> HHHHHHSSGLEVLFQGPHMASMPEQYRYTLPVKAGEQRLLGELTGAACATLVAEIAERHAGPVVLIAPDMQNALRLHDEISQFTDQMVMNLADWETLPYDSFSPHQDIISSRLSTLYQLPTMQRGVLIVPVNTLMQRVCPHSFLHGHALVMKKGQRLSRDALRTQLDSAGYRHVDQVMEHGEYATRGALLDLFPMGSELPYRLDFFDDEIDSLRVFDVDSQRTLEEVEAINLLPAHEFPTDKAAIELFRSQWRDTFEVKRDPEHIYQQVSKGTLPAGIEYWQPLFFSEPLPPLFSYFPANTLLVNTGDLETSAERFQADTLARFENRGVDPMRPLLPPQSLWLRVDELFSELKNWPRVQLKTEHLPTKAANANLGFQKLPDLAVQAQQKAPLDALRKFLETFDGPVVFSVESEGRREALGELLARIKIAPQRIMRLDEASDRGRYLMIGAAEHGFVDTVRNLALICESDLLGERVARRRQDSRRTINPDTLIRNLAELHIGQPVVHLEHGVGRYAGMTTLEAGGITGEYLMLTYANDAKLYVPVSSLHLISRYAGGAEENAPLHKLGGDAWSRARQKAAEKVRDVAAELLDIYAQRAAKEGFAFKHDREQYQLFCDSFPFETTPDQAQAINAVLSDMCQPLAMDRLVCGDVGFGKTEVAMRAAFLAVDNHKQVAVLVPTTLLAQQHYDNFRDRFANWPVRIEMISRFRSAKEQTQILAEVAEGKIDILIGTHKLLQSDVKFKDLGLLIVDEEHRFGVRHKERIKAMRANVDILTLTATPIPRTLNMAMSGMRDLSIIATPPARRLAVKTFVREYDSMVVREAILREILRGGQVYYLYNDVENIQKAAERLAELVPEARIAIGHGQMRERELERVMNDFHHQRFNVLVCTTIIETGIDIPTANTIIIERADHFGLAQLHQLRGRVGRSHHQAYAWLLTPHPKAMTTDAQKRLEAIASLEDLGAGFALATHDLEIRGAGELLGEEQSGSMETIGFSLYMELLENAVDALKAGREPSLEDLTSQQTEVELRMPSLLPDDFIPDVNTRLSFYKRIASAKTENELEEIKVELIDRFGLLPDPARTLLDIARLRQQAQKLGIRKLEGNEKGGVIEFAEKNHVNPAWLI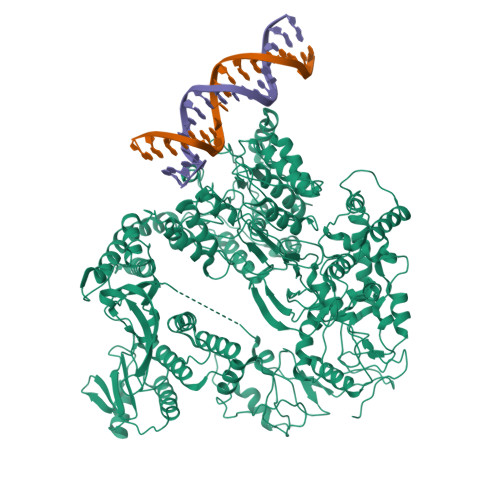GLLQKQPQHYRLDGPTRLKFIQDLSERKTRIEWVRQFMRELEENAIA> VSRDELM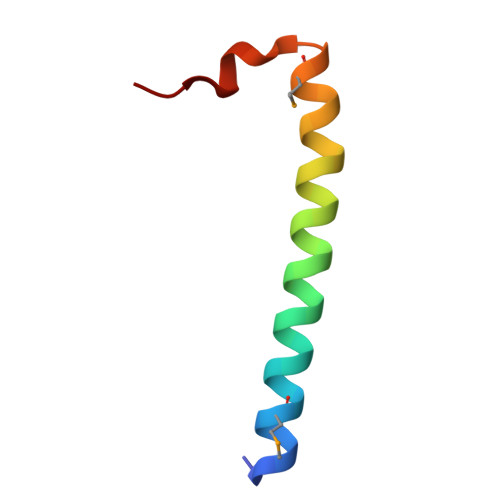EAIQKQEEINFRLQDYIDRIIVAIMETNPSILEVK> SMRKKIFKPEELRQALMPTLEALY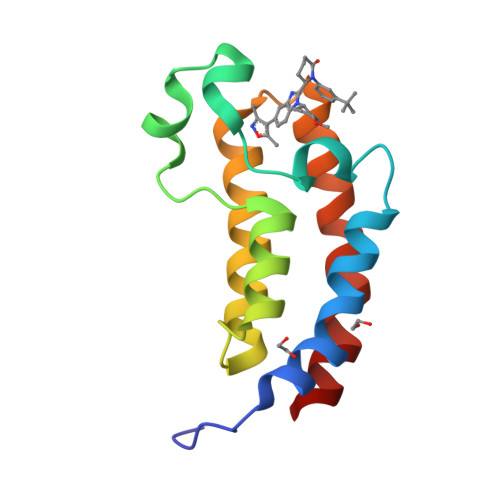RQDPESLPFRQPVDPQLLGIPDYFDIVKNPMDLSTIKRKLDTGQYQEPWQYVDDVWLMFNNAWLYNRKTSRVYKFCSKLAEVFEQEIDPVMQSLG PYROMELLITIC ACID | C10 H6 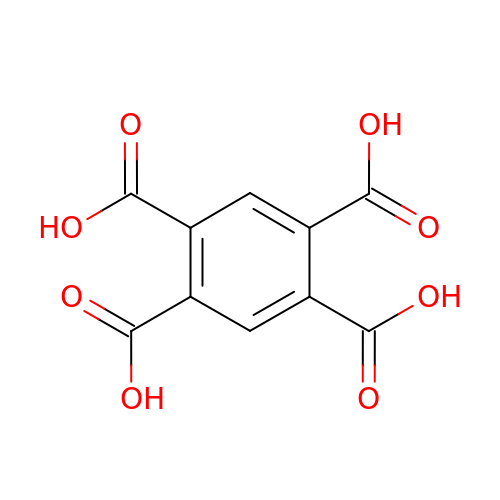O8 | CYIDZMCFTVVTJO-UHFFFAOYSA-N>GSHMTDRTDADDLDLQRVGARLAARAQIRDIRLLRTQAAVHRAPKPAQGLTYDLEFEPAVDADPATISAFVVRISCHLRIQNQAADDDVKEGDTKDETQDVATADFEFAALFDYHLQEGEDDPTEEELTAYAATTGRFALYPYIREYVYDLTGRLALPPLTLEILSRPMPVSPGAQWPATRGTP[4x];>EVPTWHRLSSYRG[3x]

Besides the generic role of SecB in protein export, SecB homologs are frequently associated (in about 7% of cases) with stress-responsive type II toxin–antitoxin (TA) systems, together forming functional tripartite TA-chaperone (TAC) systems. The human pathogen Mycobacterium tuberculosis possesses such a TA-associated SecB chaperone, named Mtb-SecBTA, which specifically controls the Mtb-HigB1 (toxin)-HigA1 (antitoxin) TA pair. We have recently shown that in contrast with chaperone-independent TA systems, the Mtb-HigA1 antitoxin of TAC possesses a C-terminal extension, named ChAD (chaperone addiction), which makes the antitoxin more aggregation-prone and renders it chaperone-dependent. In this case, the ChAD extension is specifically recognized by the Mtb-SecBTA chaperone, which protects it from both aggregation and degradation.

To investigate the SecB substrate-binding property, we have solved the structure of Mtb-SecBTA together with the short C-terminal fragment of the Mtb-HigA1 antitoxin (named ChAD), which was found as the main site of interaction with the chaperone, both in vivo and in vitro. The structure comprises a Mtb-SecBTA homotetramer (the subunits, termed A–D, contain 136–138 residues of the 181 amino acids found in the Mtb-SecBTA sequence) to which three ChAD peptides (corresponding to sequence 104EVPTWHRLSSYRG116 of Mtb-HigA1 named C4 in a previous study; subunits E–G), 2 dimethyl sulfoxide (DMSO) molecules, and 3 Ca2+ ions are bound. The three-dimensional fold of Mtb-SecBTA consists of a six-residue long N-terminal helix (αN) followed by a four-stranded antiparallel β-sheet (β1–β4), each strand contributing 13–16 residues, and a 30-residue long C-terminal helix (α1) that is prolonged by an extended peptide segment running parallel to α1. Two subunits associate through their β1 strands to form β-dimers (A–B and C–D), resulting in an eight-stranded antiparallel β-sheet. Three Ca2+ ions were localized based on electronic density and geometric criteria, and calcium binding occurs in subunits A, B, and D at the same position. Binding occurs on the thinner side of the Mtb-SecBTA chaperone tetramer. On one side, two peptides (chains E and F) are bound in a symmetrical way (related by a twofold axis) and adopt strictly the same extended conformation with a rmsd of 0.6 Å based on main-chain atoms. The third peptide (chain G) binds on the opposite side and also adopts an extended conformation identical from residues 104–108 (rmsd of 0.5 Å on backbone atoms) but differs in main-chain (φ,ψ) angles from residues 109–114 (rmsd of 2.1 Å). Each bound peptide makes contact with three protein subunits in a similar way, with some variations. In agreement with previous in vivo data, the structure reveals that three ChAD residues play a major structural role in complex formation, namely W108, R110, and Y114.> MRNQELARIFEEIGLMSEFLGDNPFRVRAYHQAARTLYDLDTPIEEIAEKGKEALMELPGVGPDLAEKILEFLRTGKVRKHEELSRKVPRGVLEVMEVPGVGPKTARLLYEGLGIDSLEKLKAALDRGDLTRLKGFGPKRAERIREGLALAQAAGK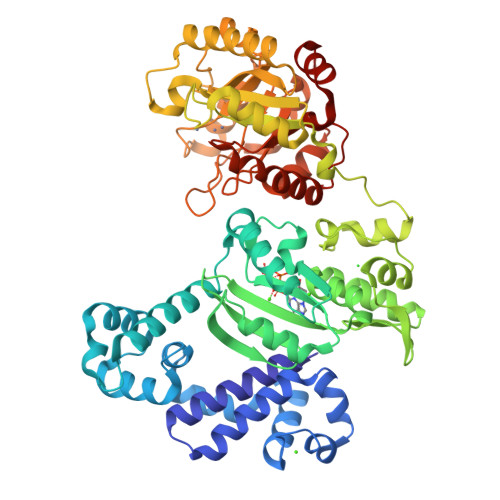RRPLGAVLSLARSLLEAIRALPGVERAELCGSARRYKDTVGDLDFLVASREGERAVEGFVRLPQVKEVYAKGKERATVFLKNGLQVDLRVVPPESYGAGLQYLTGSKAHSIRLRALAQEKGLKLSEYGVFRGEKRIAGETEEEVYAALGLPWIPPPLREDQGEVEAALEGRLPKLLELPQVKGDLQVHSTYSDGQNTLEELWEAAKTMGYRYLAVTDHSPAVRVAGGPSPEEALKRVGEIRRFNETHGPPYLLAGAEVDIHPDGTLDYPDWVLRELDLVLVSVHSRFNLPKADQTKRLLKALENPFVHVLAHPTARLLGRRAPIEADWEAVFQKAKEKGVAVEIDGYYDRMDLPDDLARMAYGMGLWISLSTDAHQTDHLRFMELAVGTAQRAWIGPERVLNTLDYEDLLSWLKARRGV> MRRTLHNELQELRGNIRVYCRIRPALKNLENSDTSLINVNEFDDNSGVQSMEVTKIQNTAQVHEFKFDKIFDQQDTNVDVFKEVGQLVQSSLDGYNVCIFAYGQTGSGKTFTMLNPGDGIIPSTISHIFNWINKLKTKGWDYKVNCEFIEIYNENIVDLLRSDNNNKEDTSIG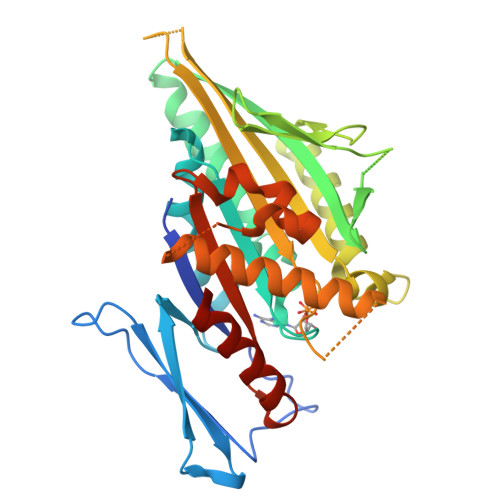LKHEIRHDQETKTTTITNVTSCKLESEEMVEIILKKANKLRSTASTASNEHSSRSHSIFIIHLSGSNAKTGAHSYGTLNLVDLAGSERINVSQVVGDRLRETQNINKSLSCLGDVIHALGQPDSTKRHIPFRNSKLTYLLQYSLTGDSKTLMFVNISPSSSHINETLNSLRFASKVNSTRLVSRK L-ALPHA-GLYCEROPHOSPHORYLSERINE 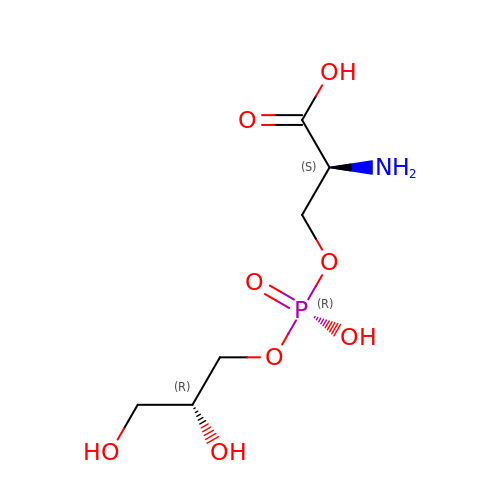| C6 H14 N O8 P | ZWZWYGMENQVNFU-UHNVWZDZSA-N[(2R)-2-{2-[hydroxy(methyl)amino]-2-oxoethyl}-5-(4-methoxyphenyl)pentyl]phosphonic acid | C15 H24 N 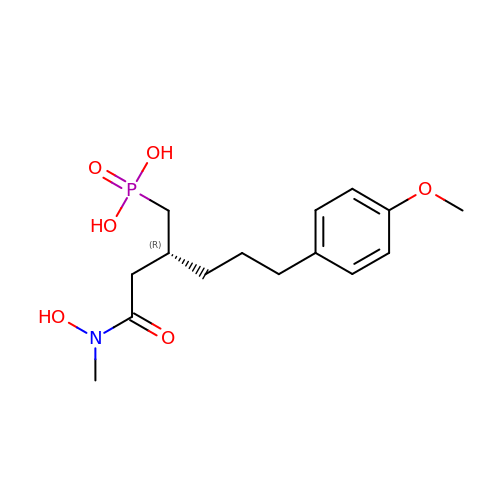O6 P | QEUMCKOMQCGMBO-CYBMUJFWSA-N>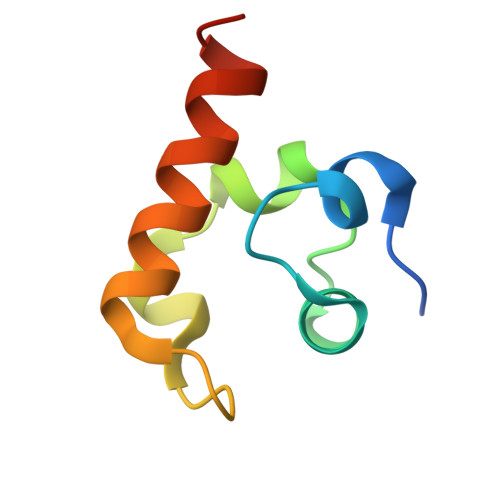 GAMDNKPADDLLNLEGVDRDLAFKLAARGVCTLEDLAEQGIDDLADIEGLTDEKAGALIMAARNICWFGDEA3-PYRIDINYLCARBINOL | C6 H7 N O | 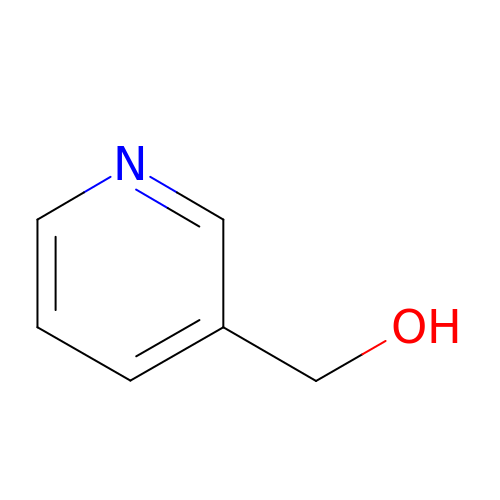MVQVNTPHUGQQHK-UHFFFAOYSA-N> MEQNPQSQLKLLVTRGKEQGYLTYAEVNDHLPEDIVDSDQIEDIIQMINDMGIQVMEEAPDADDLMLAENTADEDAAEAAAQVLSSVESEIGRTTDPVRMYMREMGTVELLTREGEIDIAKRIEDGINQVQCSVAEYPEAI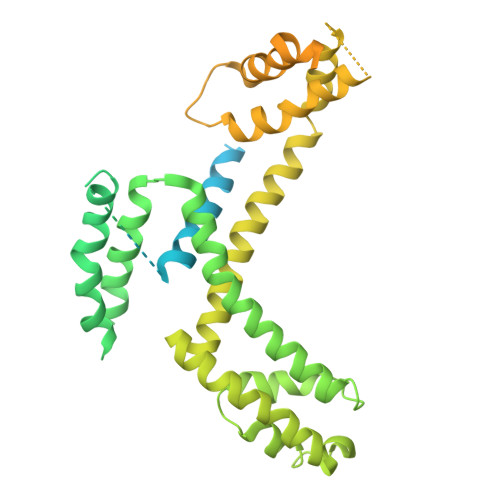TYLLEQYDRVEAEEARLSDLITGFVDPNAEEDLAPTATHVGSELSQEDLDDDEDEDEEDGDDDSADDDNSIDPELAREKFAELRAQYVVTRDTIKAKGRSHATAQEEILKLSEVFKQFRLVPKQFDYLVNSMRVMMDRVRTQERLIMKLCVEQCKMPKKNFITLFTGNETSDTWFNAAIAMNKPWSEKLHDVSEEVHRALQKLQQIEEETGLTIEQVKDINRRMSIGEAKARRAKKEMVEANLRLVISIAKKYTNRGLQFLDLIQEGNIGLMKAVDKFEYRRGYKFSTYATWWIRQAITRSIADQARTIRIPVHMIETINKLNRISRQMLQEMGREPTPEELAERMLMPEDKIRKVLKIAKEPISMETPIGDDEDSHLGDFIEDTTLELPLDSATTESLRAATHDVLAGLTAREAKVLRMRFGIDMNTDHTLEEVGKQFDVTRERIRQIEAKALRKLRHPSRSEVLRSFLDD>MNKPSFLLVGLLVVSGVLGAAETKVKYPDGFRSWYHVKSMVIQPGHPLENPVGGIHHVYANAEAIQGLRGGNYPDGAVLVFDLFDYQEDNHALVEGKRKLIGVMERDAKRFSATGGWGYEGFGEGKPDKRLVTDGGQGCFGCHAAQKESQYVFSRLRD[2x]

Cytochromes c′ (cyts c′) are a group of putative NO-binding heme proteins that fall into two families: the well-characterized four alpha helix bundle fold (cyts c′-α) and an unrelated family with a large beta-sheet fold (cyts c′-β) resembling that of cytochromes P460. Of these, cytochrome P460 (cytP460) is a heme enzyme that oxidizes hydroxylamine to N2O as part of nitrification (1), whereas the evolutionarily related cytochrome c′-β (cyt c′-β) binds the diatomic gases, NO and CO (2). By contrast, our recent crystal structure of cyt c′-β from Methylococcus capsulatus (Bath) (McCP-β) reveals a hydrophobic distal pocket dominated by two Phe residues (F32 and F61), a structural feature we have named the “Phe cap. Proposed roles for cyt c′-β proteins include protection against NO stress generated during nitrification.

We further probed the roles of the distal Phe cap residues (Phe 61 and Phe 32) by comparing the properties of wt McCP-β with those of the F32V and F61V variants, focusing on NO and CO complexes. Our goal in characterizing these aromatic → aliphatic variants was twofold: (i) to provide further evidence that the Phe 32 aromatic quadrupole limits Fe(II)→XO(π∗) backbonding and (ii) to establish the extent to which the Phe 32 aromatic quadrupole influences heme–gas reactivity. We assessed the impact of the Phe 32 aromatic quadrupole on McCP-β heme–gas affinity by comparing the structural, spectroscopic, and kinetic properties of wt McCP-β with those of the F61V and F32V variants.> GHKPEPTDEEWELIKTVTEAHVATNAQGSHWKQKRKFLPEDIGQAPIVNAPEGGKVDLEAFSHFTKIITPAITRVVDFAKKLPMFCELPCEDQIILLKGCCMEIMSLRAAVRYDPESETLTLSGEMAVTRGQLKNGGLGVVSDAIFDLGMSLSSFNLDDTEVALLQAVLLMSSDRPGLACVERIEKYQDSFLLAFEHYINYRKHHVTHFW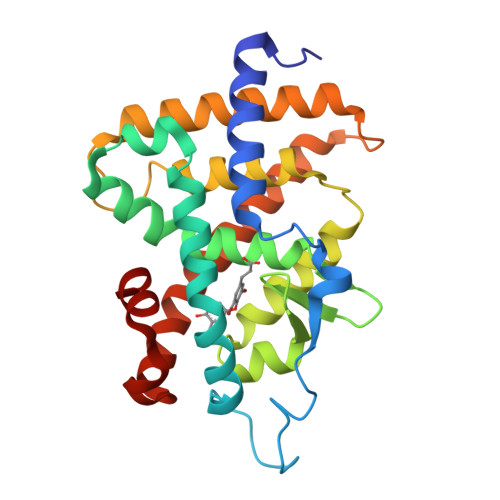PKLLMKVTDLRMIGACHASRFLHMKVECPTELFPPLFLEVFED>GSHMANKRNEALRIESALLNKIAMLGTEKTAEAV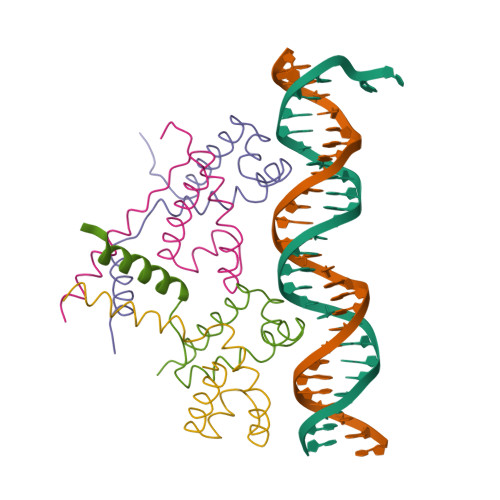GVDKSQISRWKRDWIPKFSMLLAVLEWGVVDDDMARLARQVAAILTNKK[4x]>[7x]MAIAQLATEYVFSDFLLKEPTEPKFKGLRLELAVDKMVTCIAVGLPLLLISLAFAQEISIGTQISCFSPSSFSWRQAAFVDSYCWAAVQQKNSLQSESGNLPLWLHKFFPYILLLFAILLYLPPLFWRFA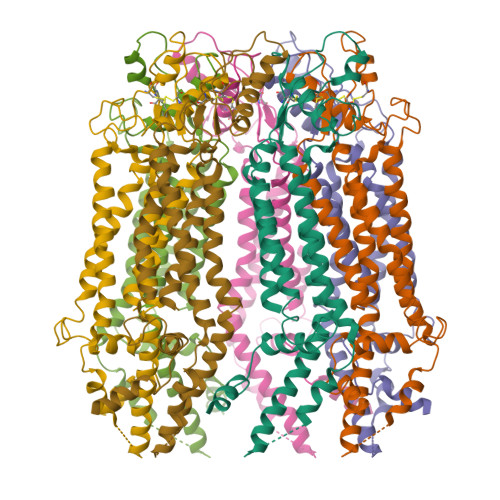AAPHICSDLKFIMEELDKVYNRAIKAAKSARDLDMRDGACSVPGVTENLGQSLWEVSESHFKYPIVEQYLKTKKNSNNLIIKYISCRLLTLIIILLACIYLGYYFSLSSLSDEFVCSIKSGILRNDSTVPDQFQCKLIAVGIFQLLSVINLVVYVLLAPVVVYTLFVPFRQKTDVLKVYEILPTFDVLHFKSEGYNDLSLYNLFLEENISEVKSYKCLKVLENIKSSGQGIDPMLLLTNLGMIKMEVVEGKTPMSAEMREEQGNQTAELQGMNIDSETKANNGEKNARQRLLDSSCGSGSHHHHHHHHHH rebaudioside D | C50 H80 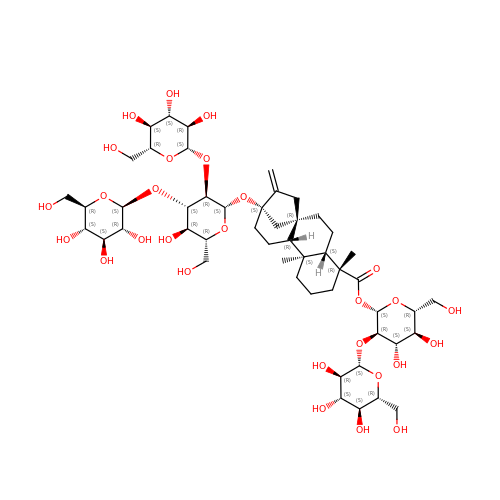O28 | RPYRMTHVSUWHSV-CUZJHZIBSA-N>[4x]MVSKGEELIKENMHSKLYLEGSVNGHQFKCTHEGEGKPYEGTQTNRIKVVEGGPLPFAFDILATMFMYGSKTF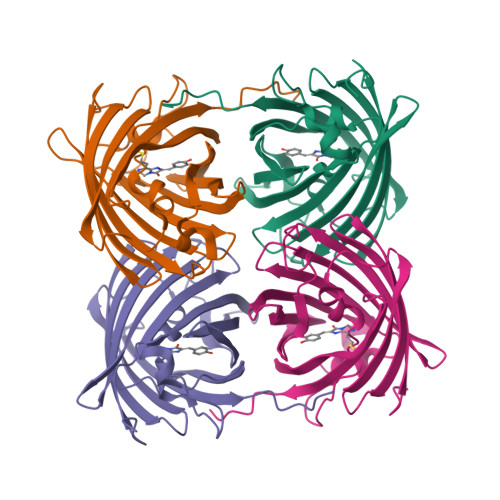IKYPKGLPDYFKQSFPEGFTWERVMVFEDGGVLTATQDTSLQDGCLIYNVKLRGVNFPANGPVMQKKTLGWEPSTETLYPADGGLEGRCDKALKLVGGGHLHCNFKTTYRSKKPATNLKMPGVHYVDRRLERIKEADNETYVEQHEVAVARYCDLPSKLGHKLNGMDELYK>[2x]MSRNNPFYFPSRRFSTRYGNQNGRIRVLQRFDQ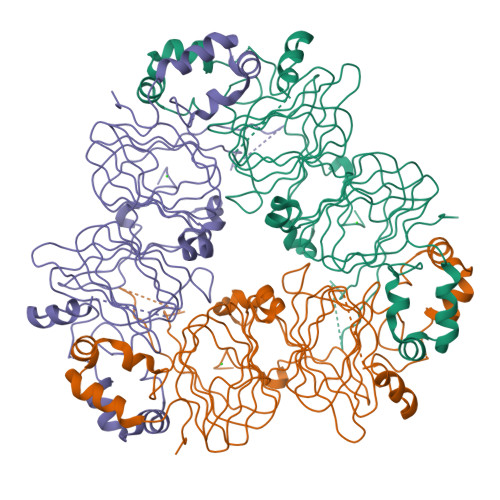RSRQFQNLQNHRIVQIEAKPNTLVLPKHADADNILVIQQGQATVTVANGNNRKSFNLDEGHALRIPSGFISYILNRHDNQNLRVAKISMPVNTPGQFEDFFPASSRDQSSYLQGFSRNTLEAAFNAEFNEIRRVLLEENAGGEQEERGQRRWSTRSSENNEGVIVKVSKEHVEELTKHAKSVSKKGSEEEGDITNPINLREGEPDLSNNFGKLFEVKPDKKNPQLQDLDMMLTCVEIKEGALMLPHFNSKAMVIVVVNKGTGNLELVAVRKEQQQRGRREEEEDEDEEEEGSNREVRRYTARLKEGDVFIMPAAHPVAINASSELHLLGFGINAENNHRIFLAGDKDNVIDQIEKQAKDLAFPGSGEQVEKLIKNQKESHFVSAR>[5x]MNESVKEIPDVLKSQCGFNCLTDISHSSFNEFRQQVSEHLSWSETHDLYHDAQQAQKDNRLYEARILKRANPQLQNAVHLAILAPNAELIGYNNQFSGRASQYVAPGTVSSMFSPAAYLTELYREARNLHASDSVYYLDTRRPDLKSMALSQQNMDIELSTLSLSNELLLESIKTESKLENYTKVMEMLSTFRPSGAT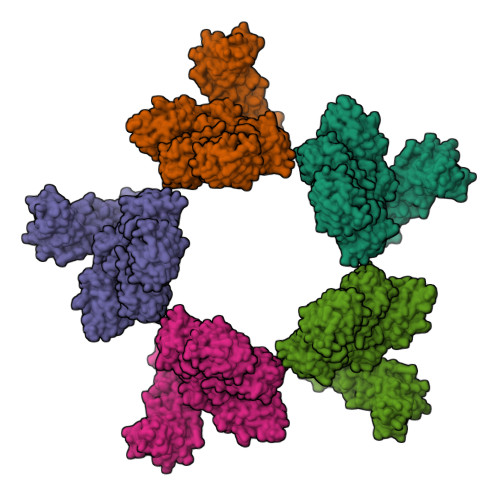PYHDAYENVREVIQLQDPGLEQLNASPAIAGLMHQASLLGINASISPELFNILTEEITEGNAEELYKKNFGNIEPASLAMPEYLKRYYNLSDEELSQFIGKASNFGQQEYSNNQLITPVVNSSDGTVKVYRITREYTTNAYQMDVELFPFGGENYRLDYKFKNFYNASYLSIKLNDKRELVRTEGAPQVNIEYSANITLNTADISQPFEIGLTRVLPSGSWAYAAAKFTVEEYNQYSFLLKLNKAIRLSRATELSPTILEGIVRSVNLQLDINTDVLGKVFLTKYYMQRYAIHAETALILCNAPISQRSYDNQPSQFDRLFNTPLLNGQYFSTGDEEIDLNSGSTGDWRKTILKRAFNIDDVSLFRLLKITDHDNKDGKIKNNLKNLSNLYIGKLLADIHQLTIDELDLLLIAVGEGKTNLSAISDKQLATLIRKLNTITSWLHTQKWSVFQLFIMTSTSYNKTLTPEIKNLLDTVYHGLQGFDKDKADLLHVMAPYIAATLQLSSENVAHSVLLWADKLQPGDGAMTAEKFWDWLNTKYTPGSSEAVETQEHIVQYCQALAQLEMVYHSTGINENAFRLFVTKPEMFGAATGAAPAHDALSLIMLTRFADWVNALGEKASSVLAAFEANSLTAEQLADAMNLDANLLLQASIQAQNHQHLPPVTPENAFSCWTSINTILQWVNVAQQLNVAPQGVSALVGLDYIQSMKETPTYAQWENAAGVLTAGLNSQQANTLHAFLDESRSAALSTYYIRQVAKAAAAIKSRDDLYQYLLIDNQVSAAIKTTRIAEAIASIQLYVNRALENVEENANSGVISRQFFIDWDKYNKRYSTWAGVSQLVYYPENYIDPTMRIGQTKMMDALLQSVSQSQLNADTVEDAFMSYLTSFEQVANLKVISAYHDNINNDQGLTYFIGLSETDAGEYYWRSVDHSKFNDGKFAANAWSEWHKIDCPINPYKSTIRPVIYKSRLYLLWLEQKEITKQTGNSKDGYQTETDYRYELKLAHIRYDGTWNTPITFDVNKKISELKLEKNRAPGLYCAGYQGEDTLLVMFYNQQDTLDSYKNASMQGLYIFADMASKDMTPEQSNVYRDNSYQQFDTNNVRRVNNRYAEDYEIPSSVSSRKDYGWGDYYLSMVYNGDIPTINYKAASSDLKIYISPKLRIIHNGYEGQKRNQCNLMNKYGKLGDKFIVYTSLGVNPNNSSNKLMFYPVYQYSGNTSGLNQGRLLFHRDTTYPSKVEAWIPGAKRSLTNQNAAIGDDYATDSLNKPDDLKQYIFMTDSKGTATDVSGPVEINTAISPAKVQIIVKAGGKEQTFTADKDVSIQPSPSFDEMNYQFNALEIDGSGLNFINNSASIDVTFTAFAEDGRKLGYESFSIPVTLKVSTDNALTLHHNENGAQYMQWQSYRTRLNTLFARQLVARATTGIDTILSMETQNIQEPQLGKGFYATFVIPPYNLSTHGDERWFKLYIKHVVDNNSHIIYSGQLTDTNINITLFIPLDDVPLNQDYHAKVYMTFKKSPSDGTWWGPHFVRDDKGIVTINPKSILTHFESVNVLNNISSEPMDFSGANSLYFWELFYYTPMLVAQRLLHEQNFDEANRWLKYVWSPSGYIVHGQIQNYQWNVRPLLEDTSWNSDPLDSVDPDAVAQHDPMHYKVSTFMRTLDLLIARGDHAYRQLERDTLNEAKMWYMQALHLLGDKPYLPLSTTWSDPRLDRAADITTQNAHDSAIVALRQNIPTPAPLSLRSANTLTDLFLPQINEVMMNYWQTLAQRVYNLRHNLSIDGQPLYLPIYATPADPKALLSAAVATSQGGGKLPESFMSLWRFPHMLENARGMVSQLTQFGSTLQNIIERQDAEALNALLQNQAAELILTNLSIQDKTIEELDAEKTVLEKSKAGAQSRFDSYGKLYDENINAGENQAMTLRASAAGLTTAVQASRLAGAAADLVPNIFGFAGGGSRWGAIAEATGYVMEFSANVMNTEADKISQSETYRRRRQEWEIQRNNAEAELKQIDAQLKSLAVRREAAVLQKTSLKTQQEQTQSQLAFLQRKFSNQALYNWLRGRLAAIYFQFYDLAVARCLMAEQAYRWELNDDSARFIKPGAWQGTYAGLLAGETLMLSLAQMEDAHLKRDKRALEVERTVSLAEVYAGLPKDNGPFSLAQEIDKLVSQGSGSAGSGNNNLAFGAGTDTKTSLQASVSFADLKIREDYPASLGKIRRIKQISVTLPALLGPYQDVQAILSYGDKAGLANGCEALAVSHGMNDSGQFQLDFNDGKFLPFEGIAIDQGTLTLSFPNASMPEKGKQATMLKTLNDIILHIRYTIK> MST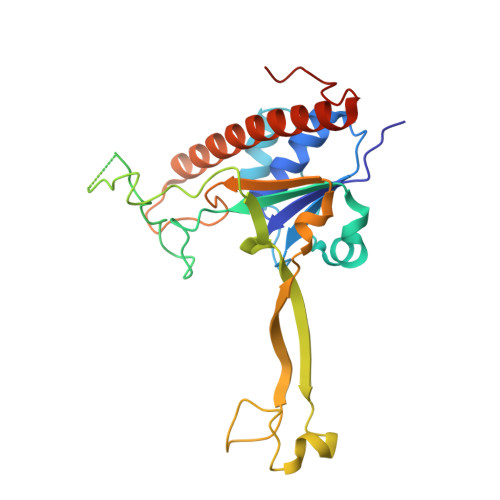SSRGILIAGLTNRARTQMAEGILRRLTAGTIFIKSGGVHHESTIHPLAVKVMKDIGIDISKQSVTSLEAARRQQNTYDVYISIDCSYERRTLDKSQPPRAEVRRRESFTVEYGDDGSGPRGGDDPVRYDPLLVPRTPSHWSVGVDATDVRRRWQIWSPRDPSIFHETSTRKFQDHLYEGEPLFMQLRQCPWRTQAKVSERWEMDEVAIRYPVERHSAHELRFVQAREQLLQRSFDLLTKLEKHYGERLLLDRALLEEFIS> MKILTQDEIEAHRSHTLKGGIEGALAGFAISAIIFKVLPRRYPKFKPSTLTWSIKTALWITPPTVLTAICAEEASNNFDATMYGSGSSSEDAL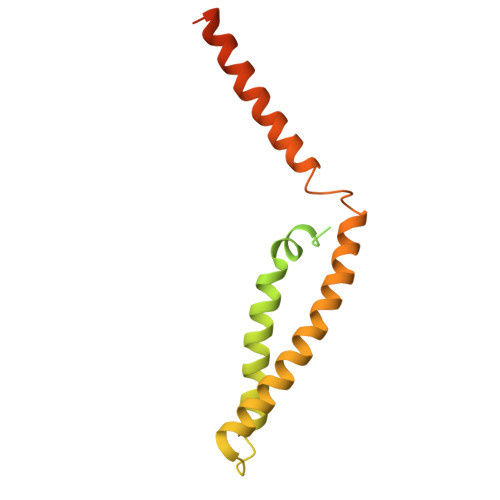DEHRRWKSLSTKDKFVEGLSNNKYKIITGAWAASLYGSWVIVNKDPIMTKAQKIVQARMYAQFITVGLLLASVGLSMYENKLHPNKQKVNEMRRWENALRVAEEEERLEKEGRRTGYVSNEERINSKIFKS>MGILRASAVHPGWPDTVGPLRVPAGVVGLRPVRMRDAAAWSRIRLADQHHLEPWEPMTGMDWKVRHAVTSWPSICSGLRAEARHGRMLPFVIELDGEFVGQLTIGNVTHGALRSAWIGYWVASSRTGGGIATAALAMGLDHCFTAVQLHRIEATVRPENTPSRAVLAHVGFREEGLLKRYLEVDGAWRDHLLVAITAEELPQSAAHRLVAAGRAEWCAA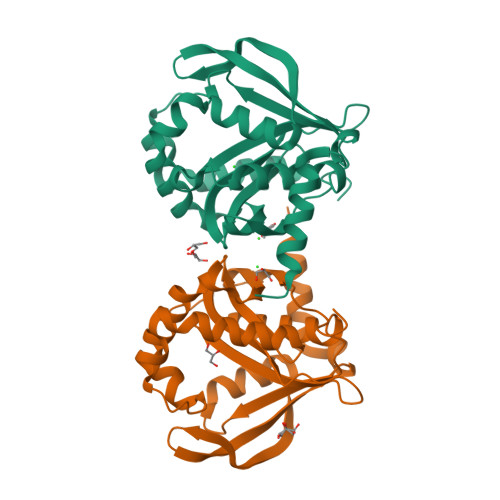A[2x]> MSLKKGKFQHNQSKSLWNYTLSPGWREEEVKILKSALQLFGIGKWKKIMESGCLPGKSIGQIYMQTQRLLGQQSLGDFMGLQIDLEAVFNQNMKKQDVLRKNNCIINTGDNPTKEERKRRIEQNRKIYGLSAKQIAEIKLPKVKKHAPQYMTLEDIENEKFTNLEILTHLYNLKAEIVRRLAEQGETIAQPSIIKSLNNLNHNLEQNQNSNSSTETKVTLEQSGKKKYKVLAIEETELQNGPIATNSQKKSINGKRKNNRKINSDSEGNEEDISLEDIDSQESEINSEEIVEDDEEDEQIEEPSKIKKRKKNPEQESEE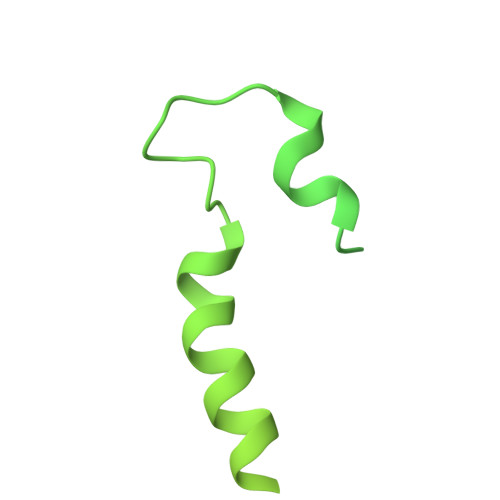DDIEEDQEEDELVVNEEEIFEDDDDDEDNQDSSEDDDDDED(2S)-2-{[2-({[(2R,3R,4R,5S,6R)-3-(acetylamino)-4,5-dihydroxy-6-(hydroxymethyl)tetrahydro-2H-pyran-2-yl]carbamothioyl}amino)ethyl](biphenyl-4-ylsulfonyl)amino}-3-methylbutanoic acid 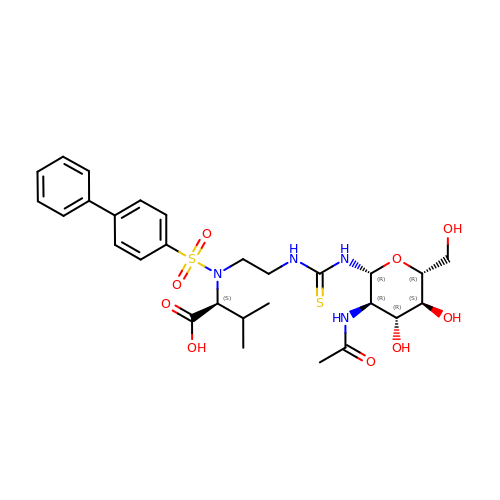(non-preferred name) | C28 H38 N4 O9 S2 | NZFBENDBEOZJMI-DIVFVBEMSA-N>[2x]MLGLKTSIIGRRVIYFQEITSTNEFAKTSYLEEGTVIVADKQTMGHGRLNRKWESPEGGLWLSIVLSPKVPQKDLPKIVFLGAVGVVETLKEFSIDGR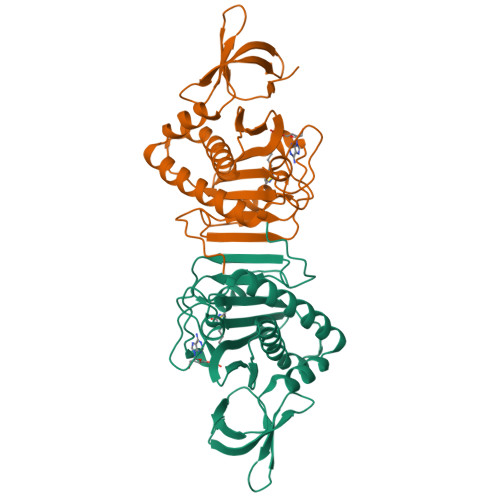IKWPNDVLVNYKGIAGVLVEGKGDKIVLGIGLNVNNKVPNGATSMKLELGSEVPLLSVFRSLITNLDRLYLNFLKNPMDILNLVRDNMILGVRVKILGDGSFEGIAEDIDDFGRLIIRLDSGEVKKVIYGDVSLRFL The IALB_1185 protein, which is encoded in the gene cluster for endo-β-1,2-glucanase homologs in the genome of Ignavibacterium album, is a glycoside hydrolase family (GH) 35 protein. Here, we showed using recombinant IALB_1185 that this protein has glycosyltransferase activity toward β-1,2-glucooligosaccharides, and that the kinetic parameters for β-1,2-glucooligosaccharides are not within the ranges for general GH enzymes. Kinetic analysis further revealed that the enzyme has wide aglycone specificity regardless of the anomer, and that the β-1,2-linked glucose dimer sophorose is an appropriate donor. We propose that IALB_1185 be redefined β-1,2-glucooligosaccharide:d-glucoside β-d-glucosyltransferase as a systematic name and β-1,2-glucosyltransferase as an accepted name.

First, we determined the ligand-free structure of wild-type IaSGT at 1.75 Å resolution after solving the initial phase by the SAD method. There are two molecules in an asymmetric unit with almost the same configuration (rsmd between subunits A and B, 0.5 Å), which is identical to the biological assembly suggested by the results of size-exclusion chromatography analysis and SDS-PAGE. In the ligand-free structure, the side chain of Arg349 is disordered beyond the Cδ atom. The side chain of Glu102 is also disordered (subunit A) or flips out from subsite −1 (subunit B). Subunit A of the ligand-free structure adopts a conformation in which both the Leu100 side chain and helix α6 are close to the substrate pocket (type 1), while subunit B adopts a conformation in which both are away from the substrate pocket (type 3). The overall conformational change on binding of ligands is small (rmsd, approximately 0.2 Å).

>[2x]MKPHNSEKYFVKNGQPHFLISGEVHYFRINPKLWRNHLQLLKQTGADTVSTYIPWDWHEIEEDDFDFEGKTHPARNLIRFIKLCKEENLDLIVKPGPYILAEYENQGLPSWLLKKLSKNAFALDENGNVISPDLVSYLSDEFLEYTFKWYDKVMPIISKHQKEHYGPITMMQLCNEIGVFQWLSGKSDYNPKVINLYKEFIIQRYKTIEKLNSVYSTNYNSFDDLKAPSGKIKLRSDYCAYFDFHLFFREYYNKYISILKNKIRSFGINIKLTHNIPGWIYGNASELPMLISTYSEIMKNHPDIIFGLDHIPEFVSFRNAHSDLACNKILEAMQPEAPVWAAEFQAGTREHHVKAYAKDLETFYIASLAHGIKGFNYYMFSQGINPEGKGFYGKTFYFQTALDAASNKLALYDSIKKVNRFIRKEQKDLLRTNVNSEICVGFYKPYFFTELISSQLLKEKKLNVEELGLYIDPRFLREEILFNGLLRGLQTLNYNYDVVDLENCDLKSLTAYKQLWITSAEFMDAETQNLLSEFVLNGGNLILYPAVPTLDNYLNRCEILKNNFGIEFITKDSSHKVSAFGIEDVFTAFSKKQIYNDTNSKPIAFTQENEICGIRKKIGKGELTILGFAFGYTSDEHLELIDKLVKLNKIKRELFVSDKDIQFVVRENNKSRYIFFLNYHNERKTFNYRKSSELKKKKSEEISIAPFSYKVIKENKLEHHHHHH methyl 2-azanylpyridine-4-carboxylate | C7 H8 N2 O2 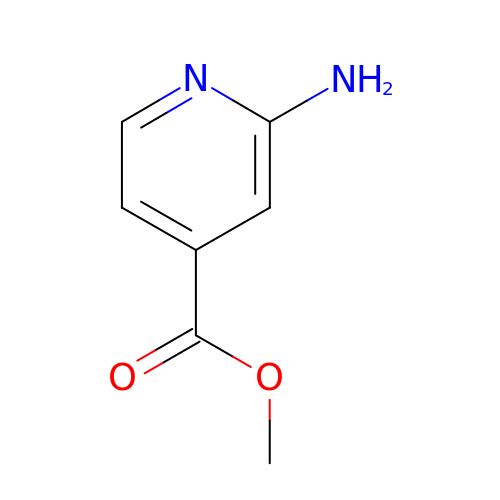| SVWWNEYBEFASMP-UHFFFAOYSA-N>[6x]AAVLFVG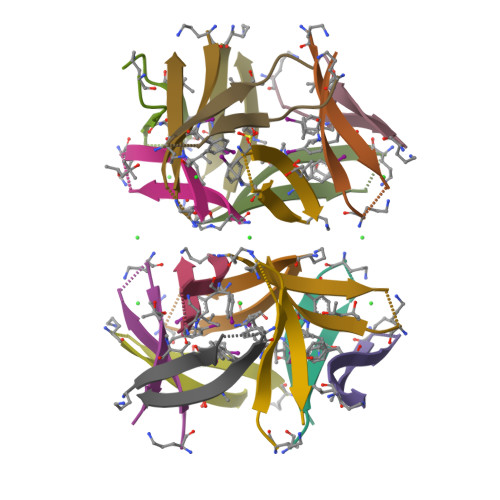SAVHGVATV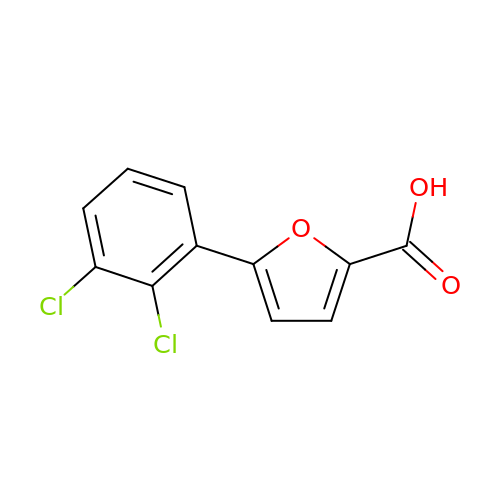5-[2,3-bis(chloranyl)phenyl]furan-2-carboxylic acid | C11 H6 Cl2 O3 | BSMKDXIJGSTBNT-UHFFFAOYSA-N In Caenorhabditis elegans (C. elegans), onset of programmed cell death is marked with the activation of CED-3, a process that requires assembly of the CED-4 apoptosome. CED-3 is synthesized as an inactive zymogen; its activation requires association with the CED-4 apoptosome. Activated CED-3 forms a holoenzyme with the CED-4 apoptosome to cleave a wide range of substrates, leading to irreversible cell death. Here, we report cryo-EM structures of the CED-4 apoptosome and three distinct CED-4/CED-3 complexes that mimic different activation stages for CED-3.

The CED-4/CED-3 catalytic complex was prepared by incubating CED-4 with a CED-3 catalytic mutant (198–503, C358A) (magenta). There were also three oligomeric states after global 3D classification, including 43.1% hexamers, 40.5% heptamers, and 16.4% octamers. In the presence of the CED-3 catalytic domain, the percentage of intact particles, that is, the heptamers and octamers, substantially increased, with the percentage of heptamers increased by about fourfolds. The 3D reconstruction of a heptamer contains a funnel-shaped density, an upper ring-like density and a globular density in the hutch. The funnel was determined to ∼ 3.6 Å resolution by applying a C7 symmetry. After local masking refinement, the resolution was improved to ∼ 6.5 Å, supporting rigid-body docking of individual CARD. The globular density in the hutch was clearly seen in both 2D and 3D classifications; however, the resolution could not be improved to support model building despite our various attempts. Six CED-4 CARDs, organized via group II stacking, and a C7 symmetric NOD funnel were resolved in the heptamer, with a height of ∼100 Å and a diameter of ∼140 Å. The heptameric architecture of NODs in the CED-4 is highly similar to that in the Apaf-1 apoptosome. Despite different oligomerization numbers, the inter-subunit interface varies little between the heptameric and octameric CED-4.

>[7x]MLCEIECRALSTAHTRLIHDFEPRDALTYLEGKNIFTEDHSELISKMSTRLERIANFLRIYRRQASELGPLIDFFNYNNQSHLADFLEDYIDFAINEPDLLRPVVIAPQFSRQMLDRKLLLGNVPKQMTCYIREYHVDRVIKKLDEMCDLDSFFLFLHGRAGSGKSVIASQALSKSDQLIGINYDSIVWLKDSGTAPKSTFDLFTDILLMLKSEDDLLNFPSVEHVTSVVLKRMICNALIDRPNTLFVFDDVVQEETIRWAQELRLRCLVTTRDVEISNAASQTCEFIEVTSLEIDECYDFLEAYGMPMPVGEKEEDVLNKTIELSSGNPATLMMFFKSCEPKTFEKMAQLNNKLESRGLVGVECITPYSYKSLAMALQRCVEVLSDEDRSALAFAVVMPPGVDIPVKLWSCVIPVDICSNEEEQLDDEVADRLKRLSKRGALLSGKRMPVLTFKIDHIIHMFLKHVVDAQTIANGISILEQRLLEIGNNNVSVPERHIPSHFQKFRRSSASEMYPKTTEETVIRPEDFPKFMQLHQKFYDSLKNFACC;>[6x]MLCEIECRALSTAHTRLIHDFEPRDALTYLEGKNIFTEDHSELISKMSTRLERIANFLRIYRRQASELGPLIDFFNYNNQSHLADFLEDYIDFAINEPDLLRPVVIAPQF Candida boidinii NAD+-dependent formate dehydrogenase (CbFDH) is a homodimeric 82 kDa enzyme complex that catalyzes the reversible conversion of formate and carbon dioxide using NAD+/NADH coenzymes for electron transfer. Candida boidinii NAD+-dependent formate dehydrogenase (CbFDH) has gained significant attention for its potential application in the production of biofuels and various industrial chemicals from inorganic carbon dioxide. Here, we present high-resolution crystal structures of apo CbFDH determined at cryogenic and ambient temperatures, as well as as that of the highly active Val120Thr mutant of CbFDH at cryogenic temperature. The inherent capability of the enzyme to catalyze the conversion of CO2 to formate holds significant potential for reducing atmospheric CO2 levels.

In CbFDH, residue 120 (Val120) is a potential mutation site for studies aiming to create a more active enzyme variant as it is located in the catalytic and substrate-binding site. The lower K m value for formate for the Val120Thr mutant indicates an approximately 1.5-fold stronger affinity for substrate binding, while the higher k cat indicates a higher turnover number (6.57-fold) compared with the wild type. The overall catalytic efficiency (k cat/K m) is found to be approximately ten times greater in the mutant CbFDH. In order to observe the effect of the Val120Thr mutation, we determined the structure of the mutant CbFDH at 1.9 Å resolution and compared it with our wild-type structure. The structure is composed of two homodimers with 99.7% completeness. Superposition of wild-type CbFDH and the Val120Thr mutant demonstrated that the overall structure does not change significantly as a consequence of this single mutation (r.m.s.d. of 0.270 Å). However, a closer look at the mutation site revealed new hydrogen bonds that does not exist in wild-type CbFDH between the threonine at position 120 and three water molecules. In the mutation site, nonetheless, we observed three new hydrogen bonds between Thr120 and water molecules in the active site. These new hydrogen bonds may help to stabilize the active site, leading to greater activity. Also, the newly formed hydrogen bonds may help to position the substrate or coenzyme molecules in the active site and contribute to a more efficient electron-transfer process during the reaction. The reason for the increase in substrate affinity may be that threonine is more polar than valine, so that it can form hydrogen bonds to neighboring amino acids or water molecules, resulting in higher stability in the substrate-binding region.

>MKIVLVLYDAGKHAADEEKLYGCTENKLGIANWLKDQGHELITTSDKEGGNSVLDQHIPDADIIITTPFHPAYITKERIDKAKKLKLVVVAGVGSDHIDLDYINQTGKKISVLEVTGSNTVSVAEHVLMTMLVLVRNFVPAHEQIINHDWEVAAIAKDAYDIEGKTIATIGAGRIGYRVLERLVPFNPKELLYYDYQALPKDAEEKVGARRVENIEELVAQADIVTINAPLHAGTKGLINKELLSKFKKGAWLVNTARGAICVAEDVAAALESGQLRGYGGDVWFPQPAPKDHPWRDMRNKYGAGNAMTPHYSGTTLDAQTRYAEGTKNILESFFTGKFDYRPQDIILLNGEYITKAYGKHDKK[4x]>[2x]YEANYEDVIKKYKPADAKLDRIAYDWRLHGGV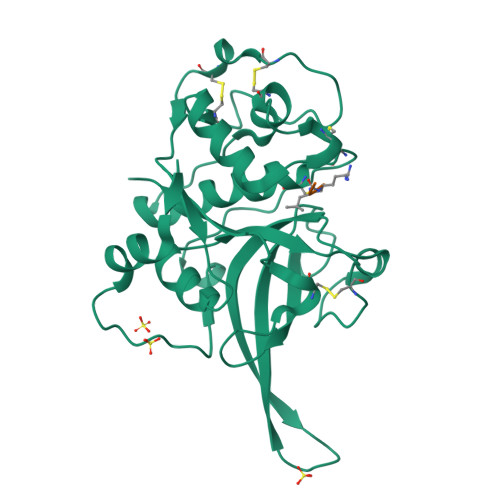TPVKDQALCGSCWAFSSVGSVESQYAIRKKALFLFSEQELVDCSVKNNGCYGGYITNAFDDMIDLGGLCSQDDYPYVSNLPETCNLKRCNERYTIKSYVSIPDDKFKEALRYLGPISISIAASDDFAFYRGGFYDGECGAAPNHAVILVGYGMKDIYNEDTGRMEKFYYYIIKNSWGSDWGEGGYINLETDENGYKKTCSIGTEAYVPLLE> MSAEREIPAEDSIKVVCRFRPLNDSEEKAGSKFVVKFPNNVEEN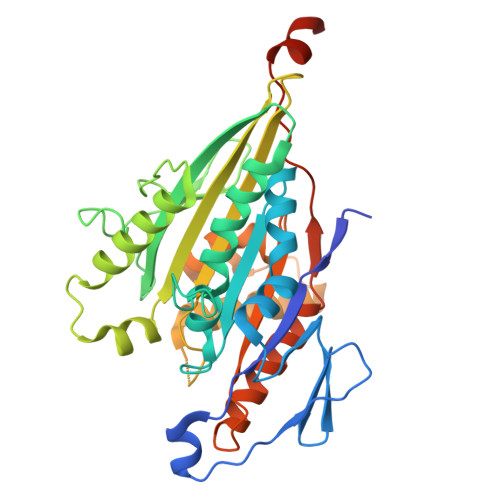CISIAGKVYLFDKVFKPNASQEKVYNEAAKSIVTDVLAGYNGTIFAYGQTSSGKTHTMEGVIGDSVKQGIIPRIVNDIFNHIYAMEVNLEFHIKVSYYEIYMDKIRDLLDVSKVNLSVHEDKNRVPYVKGATERFVSSPEDVFEVIEEGKSNRHIAVTNMNEHSSRSHSVFLINVKQENLENQKKLSGKLYLVDLAGSEKVSKTGAEGTVLDEAKNINKSLSALGNVISALADGNKTHIPYRDSKLTRILQESLGGNARTTIVICCSPASFNESETKSTLDFGRRAKTVKNVVCVNEELTAEEWKRRYEKEKEKNARLKGK Parvoviruses are linear single-stranded DNA (ssDNA) viruses with T = 1 icosahedral symmetry capsids, affecting both vertebrate and invertebrate hosts. To expand the architectural repertoire for the parvoviruses, two aveparvoviruses affecting red-crowned cranes (RCPV) or turkeys (TuPV) were selected for structural determination via cryo-EM representing two species of the genus with ~55% amino acid sequence identity comparing the VP2. The VP monomer for both aveparvoviruses retained the basic capsid architecture with the conserved eight-stranded jelly roll motif (βB–βI), which is extended by the additional βA-strand and one alpha helix (αA). Like other parvovirus capsids, the surface loops are dominated by the large GH loop, located primarily at the threefold region; the DE loop, which forms the fivefold channel pore; and the BC and EF loops, found at the two-/fivefold wall.

RCPV was first identified and characterized as part of a 2018 viral metagenomics study from the fecal virome of wild and domestic red-crowned crane populations in China. Following cryo-EM data collection, three-dimensional reconstructions of both aveparvoviruses, utilizing 405,850 RCPV and 35,131 TuPV extracted individual particles, were determined at resolutions of 2.66 Å and 2.35 Å, respectively. The short threefold protrusions of the RCPV and TuPV capsids are primarily formed by VR-IV and VR-VIII. For example, VR-IV was significantly shorter for RCPV than all other genera in Parvovirinae. These differences contribute to the truncated appearance of the threefold protrusions and fivefold pores of RCPV. With the technological advancements in recent years, cryo-EM is capable of generating high-resolution maps of macromolecules that allow us to discern fine structural details, such as water molecules or bound metal ions. Both RCPV and TuPV maps had conserved additionally ordered densities in the threefold region of the capsid, which represented potential metal-bivalent cation-binding sites (most likely Mg2+ or Ca2+) with ordered water molecules. The bivalent cation at the side of the threefold protrusion is coordinated by identical amino acids in RCPV and TuPV, including D262, T263, D272, and A273 (RCPV numbering) of VR-IV and Q355 of VR-VII. RCPV is most structurally similar to QAAV, with a structural similarity of 65%, a Dependoparvovirus which affects bob-white quails. RCPV showed robust binding to the Pro5 cells but not to the sialic acid-deficient cell line Lec2, displaying a similar binding pattern to SAAV.

>[60x]MAAADSSADAAVPMSDSPSGGGGGGGGGGIGESTGNWTCNTVWGKNSIITNASRHCVCLTRDLDMYKAIGNKDNGLVFGTENKTAWVGWSTPWNYIDYNQMCVHFSPRDWQRLINTASKWRPRSVHIKIFNIQVIQKTTVSDGTQYSNDLTGTIQIFADAQGRYPKLLYPCQTTMMGPFPNHIYYLPQYAYTTACDGPTSNQDINALLNTNSAFYCLDESPSAMLRTGNEWSCHYTFDDDTGWVHNTRSTIPIFERANPLYDTWQVDLRGNDALRGHFSSWRQPWLPGPVINMTDGTAAGANLNTMPGVDVGASYMGIVPGPPICRAENDKDEYLQTFWTPKTIGQNEGDVKNSQINTSTAYKSQVPTGRLWEVNARGQYKAASSQGNVADQQWAGCIPGMIWDRRPATYFDPIWQEKPITDDSFMYVSQMGGCTVSGAPGHIFVKNTPKPTGTANEYVDEYSTFTITVTMEWEYEPHSFSQWNNYKMISNNESSAQAYVGMCNASGQYVLNHSAGQLPEMWITKNLSRVN2-chloro-5-{[(2,2-dimethylpropanoyl)amino]methyl}-N-(1H-imidazol-2-yl)benzamide 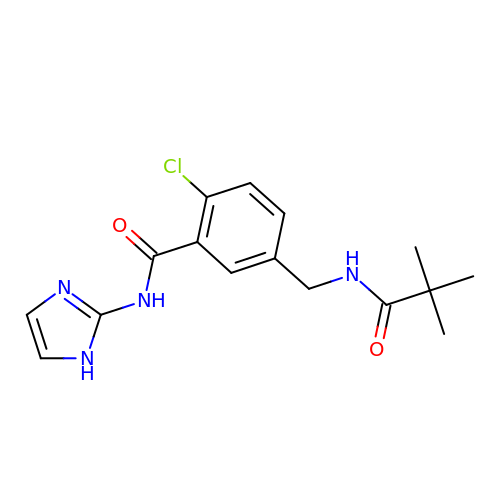| C16 H19 Cl N4 O2 | MBAHGUNQNAJTLD-UHFFFAOYSA-N>[4x]MTLTASSSSRAVTNSPVVVALDYHNRDDALAFVDKIDPRDCRLKVGKEMFTLFGPQFVRELQQRGFDIFLDLKFHDIPNTAAHAVAAA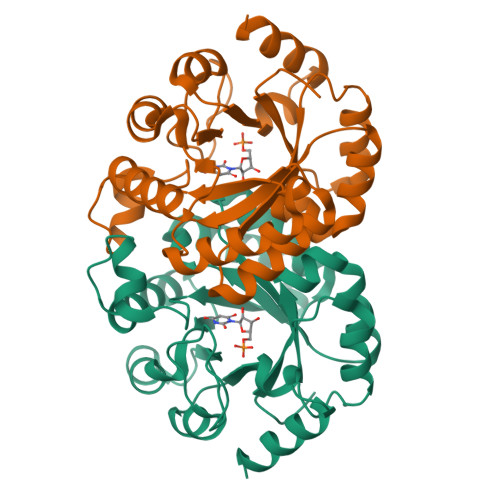ADLGVWMVNVHASGGARMMTAAREALVPFGKDAPLLIAVTVLTSMEASDLVDLGMTLSPADYAERLAALTQKCGLDGVVCSAQEAVRFKQVFGQEFKLVTPGIRPQGSEAGDQRRIMTPEQALSAGVDYMVIGRPVTQSVDPAQTLKAINASLQRSA> DAHSLWYNFTIIHLPRHGQQWCEVQSQVDQKNFLSYDCGSDKVLSMGHLEEQLYATDAWGKQLEMLREV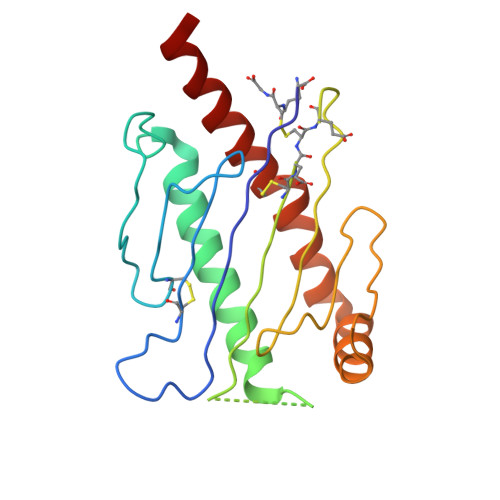GQRLRLELADTELEDFTPSGPLTLQVRMSCEXEADGYIRGSWQFSFDGRKFLLFDSNNRKWTVVHAGARRMKEKWEKDSGLTTFFKMVSMRDCKSWLRDFLMHRKKRLE> TLTEDLDAPQDTGNIENGAADNSPQPRTTFDYTGNPLPPDTKLENFFSFYRLLPMGGSGAPSLSFPADEGTIIPLDPINWLKGADVSGIAAMLSCFTYIAADLRITLRFSNPNDNPATMLVAFAPPGATIPLKPTRQMLSNFYMAEVPVSAATSTMVSFSIPYTSPLSAIPTSYFGWEDWSGTNFGQLSSGSWGNLMLIPSLSVDSAIPFDFQLSCWV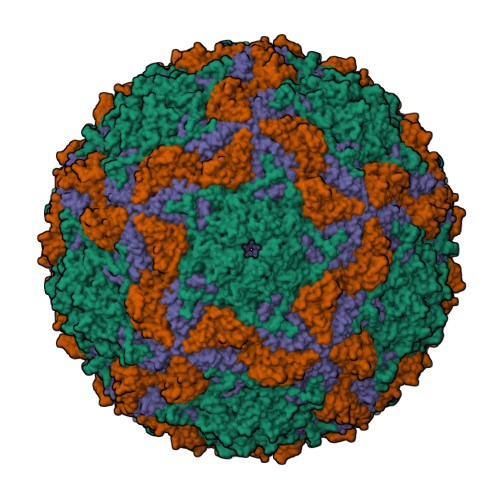AFGNFKAWVPRPPPPLPPLPTPAANAERTVAVIKQ;> TNIYGNGNNVNTDVGANGWAPTVSTGLGDGPVSCTPPTPSPGDTEVPPPRKPFTFPAPPTKSGSRFSKWWEPAAARASESATDSAIEGIDAAGKAASKAITRKLDRPAAPSSTANPQPSLIALNPSATQSGNASILTGSTAPSLLAYPTATPVPLPNPDEPSQPGPSGDRTWLLDTVTWSQEFTRGWNIAGSNGMQWTGLESLIFPVSTDTNWTSTSSPTAYPLPFSFVRAYPDSSWAAMYNTHSMWNCGWRVQVTVNGSQFHAGALILYMVPEATTHAIQTARDNAGFVFPYVILNLYESNTATIEVPYISPTPNTSSGLHAPWTFYLQVLSPLNPPPSLPTSLSCSIYVTPVDSSFHGLRYLAPQ;> HWKTRAVPGAGTFGSAVAGQELPLCGVRAYYPPNAYIPAQVRDWLEFAHRPGLMATVPWTMADEPAERLGIFPVSPSAIAGTGAPISYVISLFSQWRGELAAHLLFTGSAQHYGRLVVCYTPAAPQPPSTMQEAMRGTYTVWDVNAASTLEFTIPFISNSYWKTVDVNNPDALLSTTGYVSIWVQNPLVGPHTAPASALVQAFISAGESFNVRLMQNPALTS The superkiller (SKI) complex is the cytoplasmic co-factor and regulator of the RNA-degrading exosome. In human cells, the SKI complex functions mainly in co-translational surveillance-decay pathways, and its malfunction is linked to a severe congenital disorder, the trichohepatoenteric syndrome. SKIV2L activity has now been shown to act primarily in exosome-mediated degradation during co-translational mRNA surveillance pathways (Tuck et al., 2020) by extracting mRNA from stalled 80S ribosomes (Zinoviev et al., 2020). For clarity, we will refer to the human orthologs of the yeast Ski complex subunits as hSKI2 (SKIV2L, ∼137.8 kDa), hSKI3 (TTC37, ∼175.5 kDa) and hSKI8 (WDR61, ∼33.6 kDa).

To recapitulate this scenario in our system, we reconstituted an 80S-CrPV-IRES assembly with wild-type hSKI, incubated with ATP for 15 min and collected cryo-EM data on a Titan Krios microscope. In the corresponding reconstruction, the interaction between 80S and hSKI2 is essentially unchanged with respect to that observed in the presence of a prehydrolytic ATP mimic. Importantly, a fraction of the particles showed no ordered density at the base of hSKI2cat for the entire gatekeeping module. Unlike hSKI in isolation, this alignment was dominated by the ribosome-bound hSKI2 in the open state, leaving the separate hSKI gatekeeping module unresolved. The cryo-EM reconstruction of the open state shows that the RNA in the helicase channel extends with well-defined density for three nucleotides more at the 3′ end (N7, N8, and N9) than detected in the closed state. The base and sugar of ribonucleotide N7 makes polar and stacking interactions with RecA1, resulting in a twist of the ribonucleotide chain of ∼180°. The RNA 3′ end exits the helicase core in a bent conformation, with nucleotides N8 and N9 making only minor interactions with the ratchet helix. Thus, when hSKI is in the open state as observed in the active assembly, the 3′ end of the ribosome-bound RNA traverses the helicase core and occupies the space where the wedge of the gatekeeping module was bound in the closed state. Concomitantly, the density for the IRES structure disappears, suggesting that the PKs unfold as the ribosome-bound RNA is extracted and ejected by the hSKI2 helicase. The RNA-binding mode observed in the open state of hSKI and, in particular, the bent conformation, with which the ribonucleotide chain traverses the RNA exit channel of hSKI2, are similar in conformation to those observed in the structure of the exosome-bound MTR4 (Weick et al., 2018).

> MMETERLVLPPPDPLDLPLRAVELGCTGHWELLNLPGAPESSLPHGLPPCAPDLQQEAEQLFLSSPAWLPLHGVEHSARKWQRKTDPWSLLAVLGAPVPSDLQAQRHPTTGQILGYKEVLLENTNLSATTSLSLRRPPGPASQSLWGNPTQYPFWPGGMDEPTITDLNTREEAEEEIDFEKDLLTIPPGFKKGMDFAPKDCPTPAPGLLSLSCMLEPLDLGGGDEDENEAVGQPGGPRGDTVSASPCSAPLARASSLEDLVLKEASTAVSTPEAPEPPSQEQWAIPVDATSPVGDFYRLIPQPAFQWAFEPDVFQKQAILHLERHDSVFVAAHTSAGKTVVAEYAIALAQKHMTRTIYTSPIKALSNQKFRDFRNTFGDVGLLTGDVQLHPEASCLIMTTEILRSMLYSGSDVIRDLEWVIFDEVHYINDVERGVVWEEVLIMLPDHVSIILLSATVPNALEFADWIGRLKRRQIYVISTVTRPVPLEHYLFTGNSSKTQGELFLLLDSRGAFHTKGYYAAVEAKKERMSKHAQTFGAKQPTHQGGPAQDRGVYLSLLASLRTRAQLPVVVFTFSRGRCDEQASGLTSLDLTTSSEKSEIHLFLQRCLARLRGSDRQLPQVLHMSELLNRGLGVHHSGILPILKEIVEMLFSRGLVKVLFATETFAMGVNMPARTVVFDSMRKHDGSTFRDLLPGEYVQMAGRAGRRGLDPTGTVILLCKGRVPEMADLHRMMMGKPSQLQSQFRLTYTMILNLLRVDALRVEDMMKRSFSEFPSRKDSKAHEQALAELTKRLGALEEPDMTGQLVDLPEYYSWGEELTETQHMIQRRIMESVNGLKSLSAGRVVVVKNQEHHNALGVILQVSSNSTSRVFTTLVLCDKPLSQDPQDRGPATAEVPYPDDLVGFKLFLPEGPCDHTVVKLQPGDMAAITTKVLRVNGEKILEDFSKRQQPKFKKDPPLAAVTTAVQELLRLAQAHPAGPPTLDPVNDLQLKDMSVVEGGLRARKLEELIQGAQCVHSPRFPAQYLKLRERMQIQKEMERLRFLLSDQSLLLLPEYHQRVEVLRTLGYVDEAGTVKLAGRVACAMSSHELLLTELMFDNALSTLRPEEIAALLSGLVCQSPGDAGDQLPNTLKQGIERVRAVAKRIGEVQVACGLNQTVEEFVGELNFGLVEVVYEWARGMPFSELAGLSGTPEGLVVRCIQRLAEMCRSLRGAARLVGEPVLGAKMETAATLLRRDIVFAASLYTQ> MDYKDDDDKENLYFQSMPGSAAKGSELSE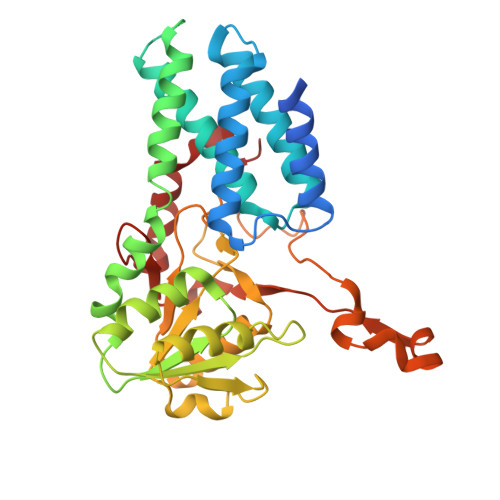RIESFVETLKRGGGPRSSEEMARETLGLLRQIITDHRWSNAGELMELIRREGRRMTAAQPSETTVGNMVRRVLKIIREEYGRLHGRSDESDQQESLHKLLTSGGLNEDFSFHYAQLQSNIIEAINELLVELEGTMENIAAQALEHIHSNEVIMTIGFSRTVEAFLKEAARKRKFHVIVAECAPFCQGHEMAVNLSKAGIETTVMTDAAIFAVMSRVNKVIIGTKTILANGALRAVTGTHTLALAAKHHSTPLIVCAPMFKLSPQFPNEEDSFHKFVAPEEVLPFTEGDILEKVSVHCPVFDYVPPELITLFISNIGGNAPSYIYRLMSELYHPDDHVL>[2x]PKIVVVGAVAGGATCASQIRRLDKESDIIIFEKDRDMSFANCALPYVIGEVVEDRRYALAYTPEKFYDRKQITVKTYHEVIAINDERQTVSVLNRKTNEQFEESYDKLILSPGASANSLGFESDITFTLRNLEDTDAIDQFIKANQVDKVLVVGAGYVSLEVLENLYERGLHPTLIHRSDKINKLM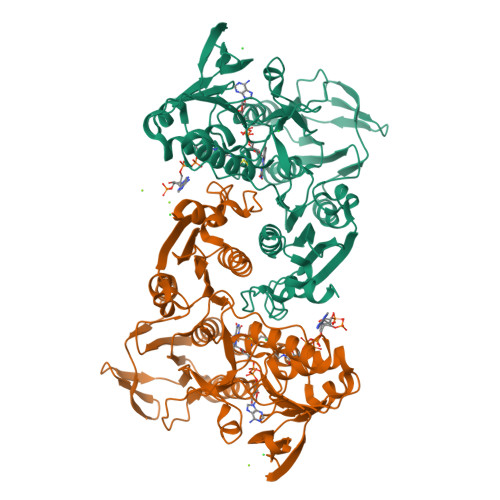DADMNQPILDELDKREIPYRLNEEINAINGNEITFKSGKVEHYDMIIEGVGTHPNSKFIESSNIKLDRKGFIPVNDKFETNVPNIYAIGDIATSHYRHVDLPASVPLAWGAHRAASIVAEQIAGNDTIEFKGFLGNNIVKFFDYTFASVGVKPNELKQFDYKMVEVTQGAHANYYPGNSPLHLRVYYDTSNRQILRAAAVGKEGADKRIDVLSMAMMNQLTVDELTEFEVAFAPPYSHPKDLINMIGYKAK> MPFEIVFEGAKEFAQLIDTASKLIDEAAFKVTEDGISMRAMDPSRVVLIDLNLPSSIFS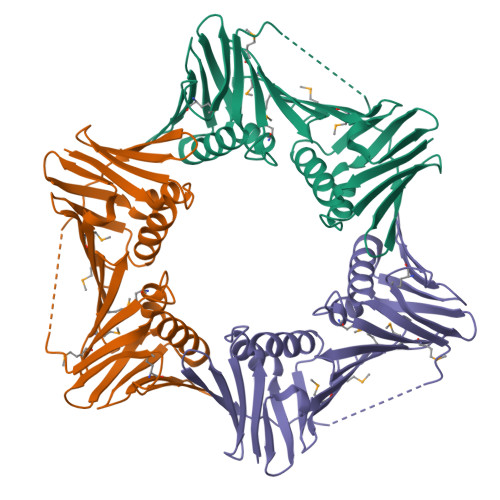KYEVVEPETIGVNLDHLKKILKRGKAKDTLILKKGEENFLEITIQGTATRTFRVPLIDVEEMEVDLPELPFTAKVVVLGEVLKDAVKDASLVSDSIKFIARENEFIMKAEGETQEVEIKLTLEDEGLLDIEVQEETKSAYGVSYLSDMVKGLGKADEVTIKFGNEMPMQMEYYIRDEGRLTFLLAPRVEE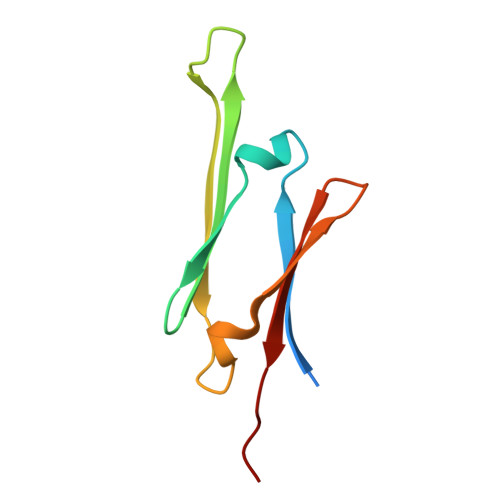> GSKFSSDASKVVTRGPGLSQAFVGQKNSFTVDCSKAGTNMMMVGVHGPKTPCEEVYVKHMGNRVYNVTYTVKEKGDYILIVKWGDESVPGSPFKVKVP;> GSGNIKTLGDAYEFAVDVRDFSPEDIIVTTSNNHIEVRAEKLAADGTVMNTFAHKSQLPEDVDPTSVTSALREDGSLTIRARRHPHT>[2x]GPLGSDLIQDVIRRAQENKQRIVLPEGLEPRTLEAADRLMADKVVNIILIGNVDSVKAKVAELGLKNLDEAVIIDPNNHPKKQQYTDLLLQIRQKKGLTPEKAAELVE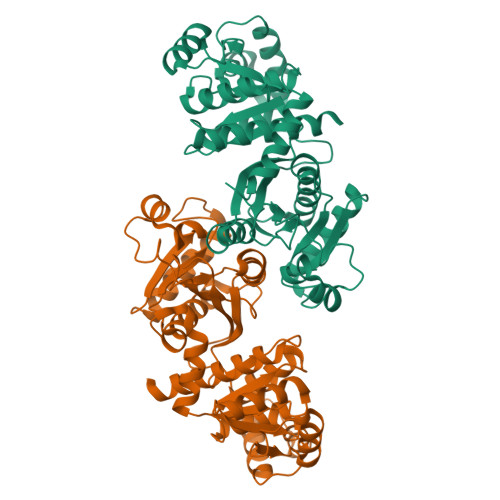NPLYLGCLIVKSGDADGLIAGAQNTTGDVLRPALQVIKTAPGMTSVSGTFLLFTKAKEYGKDGLLLVADCAVIPNPTADELAQIAVATARTAKAIADIEPRVAMLSFSTKGSAKHEMTDKVVEATRMAQEMAPDLLIDGEMQADAALVERVAALKAPGSNVAGKANVLVFPTLEVGNIAYKLVERLGHAEAVGPILQGMAAPVNDLSRGCSVEDIYRMVAITANQAIAAKEQ> LTATVDGIIQPMLKAYRIPGMAVAVLKDGKAHYFNYGVANRESGQRVSEQTLFEIGSVSKTLTATLGAYAAVKGGFELDDKVSQHAPWLKGSAFDGVTMAELATYSAGGLPLQFPDEVDSNDKMQTYYRSWSPVYPAGTHRQYSNPSIGLFGHLAANSLGQPFEQLMSQTLLPKLGLHHTYIQVPESAMANYAYGYSKEDKPIRATPGVLAAEAYGIKTGSADLLKFVEANMGYQGDAALKSAIALTHTGFHSVGEMTQGLGWESYDYPVTEQVLLAGNSPAVSFQANPVTRFAVPKAMGEQRLYNKTGSTGGFGAYVAFVPARGIAIVMLANRNYPIEARVKAAHAILSQLAE;> PLTATVDGIIQPMLKAYRIPGMAVAVLKDGKAHYFNYGVANRESGQRVSEQ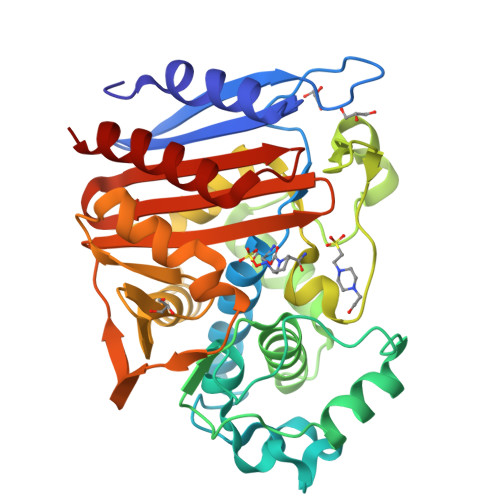TLFEIGSVSKTLTATLGAYAAVKGGFELDDKVSQHAPWLKGSAFDGVTMAELATYSAGGLPLQFPDEVDSNDKMQTYYRSWSPVYPAGTHRQYSNPSIGLFGHLAANSLGQPFEQLMSQTLLPKLGLHHTYIQVPESAMANYAYGYSKEDKPIRATPGVLAAEAYGIKTGSADLLKFVEANMGYQGDAALKSAIALTHTGFHSVGEMTQGLGWESYDYPVTEQVLLAGNSPAVSFQANPVTRFAVPKAMGEQRLYNKTGSTGGFGAYVAFVPARGIAIVMLANRNYPIEARVKAAHAILSQLAE> AASGSALIFDEEMSRYKLLWTDPECEIEVPERLTVSYEALRTHGLAQRCKAVPVRQATEQEILLAHSEEYLEAVKQTPGMNVEELMAFSKKYNAVYFHQNIYHCAKLAAGATLQLVDSVMKREVRNGMALVRPPGHHSQRSAANGFCVFNNVAFAALYAKKNYNLNRILIVDWDVHHGQGIQYCFEEDPSVLYFSWHRYEHQSFWPNLPESDYSSVGKGKGSGFNINLPWNKVGMTNSDYLAAFFHVLLPVAYEFDPELVIVSAGFDSAIGDPEGEMCALPEIFAHLTHLLMPLAAGKMCVVLEGGYNLTSLGQSVCQTVHSLLGDPTPRISGLGTACDSALESIQNVRNVQSSYWSSFKHLAQSETNPKRPRLDATNGGPKESSEPASESNPKKTAQDIVWPEPLKRMPASVRTVVVPPPGVELTLPKNCQHSGDISESTAKEVQRIRDKHFHDLTDQNILRSLGNIISVLDRMMRSDEVCNGCVVVSDLSVSVQCALQHALTEPAERV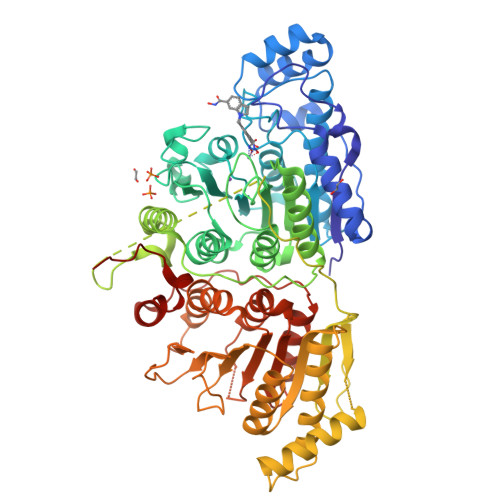LVVYVGDGELPVKTNDGKVFLVQICTKETEDKCVNRLTLCLREGESLTAGFMQALLGLILPVAYEFNPALVLGIVEETAAKTRLMRVWGHMTCLIQGLARGRMLTLLQGYDKDLLELTVSALSGASISPLGPLRAPKPEDVEMMEKQRQRLQERWGLLRCTVSESW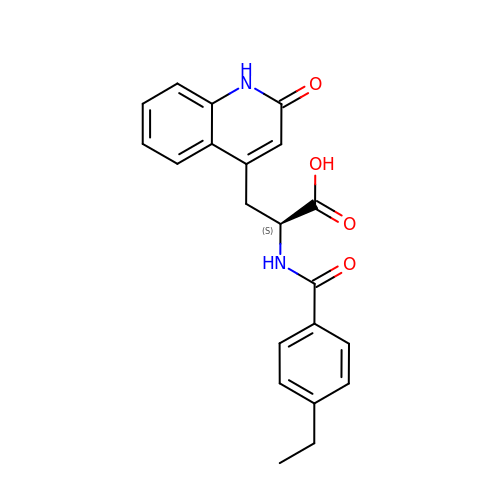N-(4-ethylbenzoyl)-3-(2-oxo-1,2-dihydroquinolin-4-yl)-L-alanine | C21 H20 N2 O4 | MOLLEYXWWDYLEA-SFHVURJKSA-N> GLVPRGSHMMEILRGSPALSAFRINKLLARFQAANLQVHNIYAEYVHFADLNAPLNDSEQAQLTRLLQYGPALSSHTPAGKLLLVTPRPGTISPWSSKATDIAHNCGLQQVDRLERGVAYYIEASTLTAEQWRQVAAELHDRMMETVFSSLTDAEKLFIHHQPAPVSSVDLLGEGRQALIDANLRLGLALAEDEIDYLQEAFTKLGRNPNDIELYMFAQANSEHCRHKIFNADWIIDGKPQPKSLFKMIKNTFETTPDYVLSAYKDNAAVMEGSAVGRYFADHNTGRYDFHQEPAHILMKVETHNHPTAISPWPGAATGSGGEIRDEGATGRGAKPKAGLVGFSVSNLRIPGFEQPWEEDFGKPERIVTALDIMTEGPLGGAAFNNEFGRPALTGYFRTYEEKVNSHNGEELRGYHKPIMLAGGIGNIRADHVQKGEIVVGAKLIVLGGPAMNIGLGGGAASSMASGQSDADLDFASVQRDNPEMERRCQEVIDRCWQLGDANPILFIHDVGAGGLSNAMPELVSDGGRGGKFELRDILSDEPGMSPLEIWCNESQERYVLAVAADQLPLFDELCKRERAPYAVIGDATEEQHLSLHDNHFDNQPIDLPLDVLLGKTPKMTRDVQTLKAKGDALNRADITIADAVKRVLHLPTVAEKTFLVTIGARTVTGMVARDQMVGPWQVPVADCAVTTASLDSYYGEAMSIGERAPVALLDFAASARLAVGEALTNIAATQIGDIKRIKLSANWMAAAGHPGEDAGLYDAVKAVGEELCPQLGLTIPVGKDSMSMKTRWQEGNEQREMTSPLSLVISAFARVEDVRHTLTPQLSTEDNALLLIDLGKGHNALGATALAQVYRQLGDKPADVRDVAQL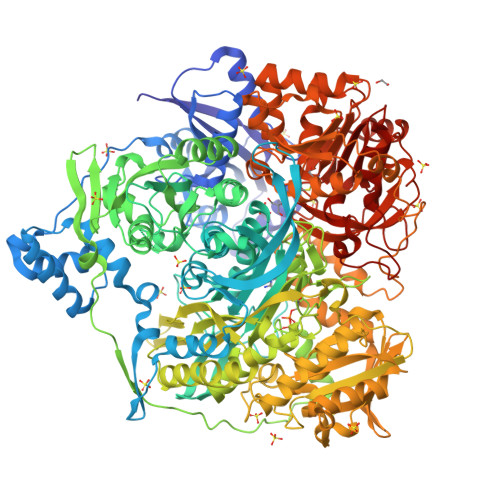KGFYDAMQALVAARKLLAWHDRSDGGLLVTLAEMAFAGHCGVQVDIAALGDDHLAALFNEELGGVIQVRAEDRDAVEALLAQYGLADCVHYLGQALAGDRFVITANDQTVFSESRTTLRVWWAETTWQMQRLRDNPQCADQEHEAKANDTDPGLNVKLSFDINEDIAAPYIATGARPKVAVLREQGVNSHVEMAAAFHRAGFDAIDVHMSDLLGGRIGLGNFHALVACGGFSYGDVLGAGEGWAKSILFNHRVRDEFETFFHRPQTLALGVCNGCQMMSNLRELIPGSELWPRFVRNHSDRFEARFSLVEVTQSPSLLLQGMVGSQMPIAVSHGEGRVEVRDDAHLAALESKGLVALRYVDNFGKVTETYPANPNGSPNGITAVTTENGRVTIMMPHPERVFRTVANSWHPENWGEDSPWMRIFRNARKQLG>[2x]MALFFRTRDRPLRPGDPYPLGSNWIEDDDGVNFSLFSENAEKVELLLYSLTNQKYPKEIIEVKNKTGDIWHVFVPGLRPGQLYAYRVYGPYKPELGLRFNPNKVLIDPYAKAINGSVIWNDAVFGYKIGDQNQDLTYDERDSGEYVPKSVVINPYFEWDDEDFIKGKKVPLKDTVIYEVHVKGFTKLRLDLPENIRGTYEGLASEQMISYLKDLGITTVELMPVFHFIDQRFLTDKGLTNYWGYDPINFFSPECRYSSTGCLGGQVLSFKKMVNELHNAGIEVIIDVVYNHTAEGNHLGPTLSFRGIDNTAYYMLQPDNKRYYLDFTGTGNTLNLSHPRVIQMVLDSLRYWVTEMHVDGFRFDLAAALARELYSVNMLNTFFIALQQDPILSQVKLIAEPWDVGQGGYQVGNFPYQWAEWNGKYRDSIRRFWRGEALPY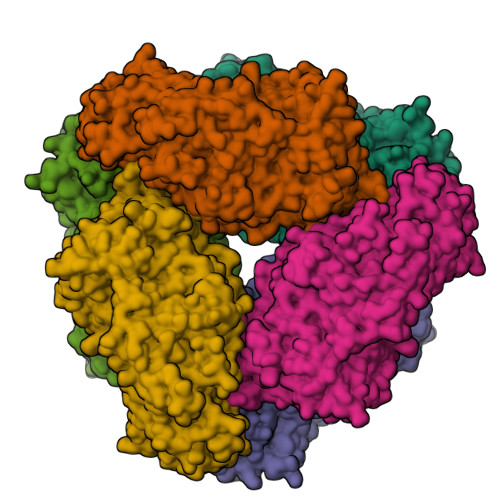SEIANRLLGSPDIYLGNNKTPFASINYVTSHDGFTLEDLVSYNQKHNEANGFNNQDGMNENYSWNCGAEGPTNDQNVVICREKQKRNFMITLLVSQGTPMILGGDELSRTQRGNNNAFCQDNEITWFDWNLDERKSKFLEFVKKMIQFYRAHPAFRRERYFQGKKLFGMPLKDVTFYTLEGREVDEKTWSSPTQLVIFVLEGSVMDEINMYGERIADDSFLIILNANPNNVKVKFPKGKWELVISSYLREIKPEERIIEGEKELEIEGRTALVYRRIEL> 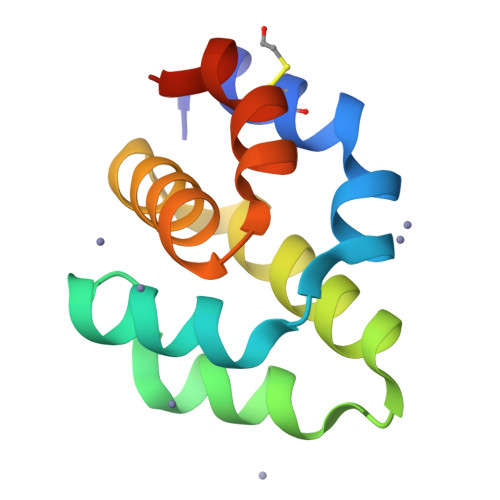MDAKARNCLLQHREALEKDIKTSYIMDHMISDGFLTISEEEKVRNEPTQQQRAAMLIKMILKKDNDSYVSFYNALLHEGYKDLAALLHDGIPVVSSS> MTENILRKSDEEIQKEITARVKALESMLIEQGILTTSMIDRMAEIYENEVGPHLGAKVVVKAWTDPEFKKRLLADGTEACKELGIGGLQGEDMMWVENTDEVHHVVVCTLCSC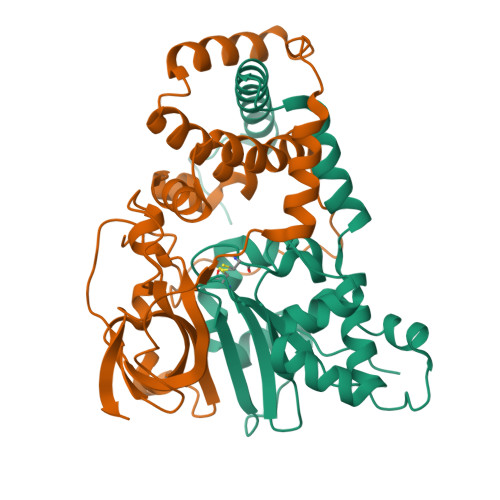YPWPVLGLPPNWFKEPQYRSRVVREPRQLLKEEFGFEVPPSKEIKVWDSSSEMRFVVLPQRPAGTDGWSEEELATLVTRESMIGVEPAKAV;> MNGVYDVGGTDGLGPINRPADEPVFRAEWEKVAFAMFPATFRAGFMGLDEFRFGIEQMNPAEYLESPYYWHWIRTYIHHGVRTGKIDLEELERRTQYYRENPDAPLPEHEQKPELIEFVNQAVYGGLPASREVDRPPKFKEGDVVRFSTASPKGHAKRARYVRGKTGTVVKHHGAYIYPDTAGNGLGECPEHLYTVRFTAQELWGPEGDPNSSVYYDCWEPYIELVDT1-O-phosphono-alpha-D-xylopyranose 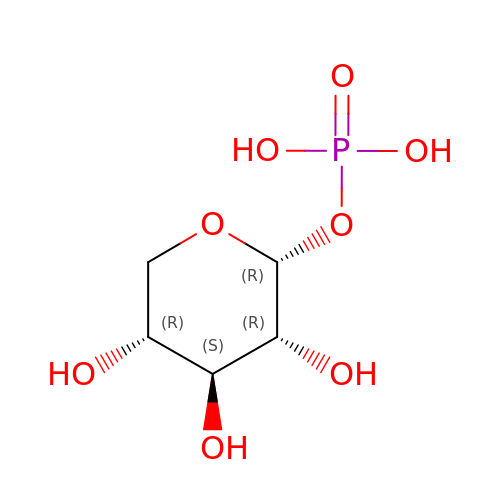| C5 H11 O8 P | ILXHFXFPPZGENN-KKQCNMDGSA-N>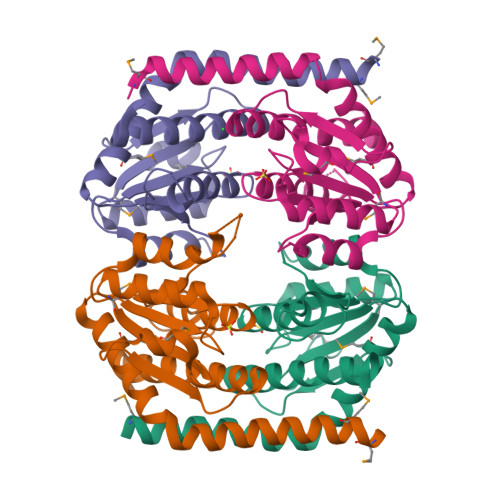GHMDMQHRIRQLFQASIETKQQALEVLPPYIEQASLVMVNALLNEGKILSCGNGGSAGDAQHFSSELLNRFERERPSLPAVALTTDSSTITSIANDYSYNEVFSKQIRALGQPGDVLLAISTSGNSANVIQAIQAAHDREMLVVALTGRDGGGMASLLLPEDVEIRVPSKITARIQEVHLLAIHCLCDLIDRQLFGSEE[4x]> 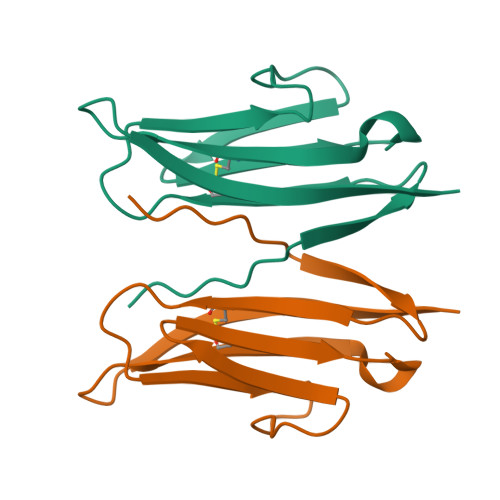LQVTISLSKVELSVGESKFFTCTAIGEPESIDWYNPQGEKIISTQRVVVQKEGVRSRLTIYNANIEDAGIYRCQATDAKGQTQEATVVLEIYQ> TGKAWCCTVLSAFGVVILSVIAHLFNTNHESFVGSINDPEDGPAVA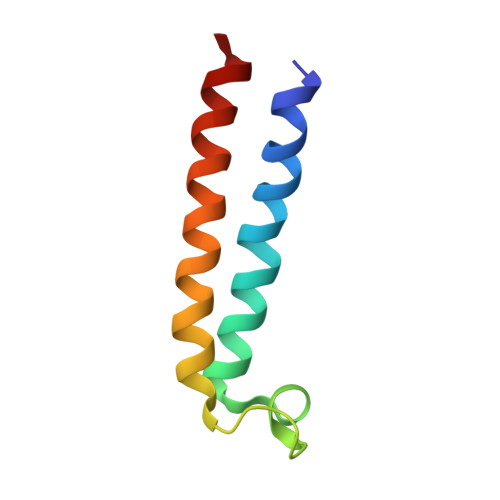HTVYLAALVYLVFFVFCGFQVYL>[2x]YYDYDHGSLGEPIRGVNIGGWLLLEPYITPSLFEAFRTNDDNDEGIPVDEYHFCQYLGKDLAKSRLQSHWSTFYQEQDFANIASQGFNLVRIPIGYWAFQILDDDPYVSGLQESYLDQAIGWARNNSLKVWVDLHGAAGSQN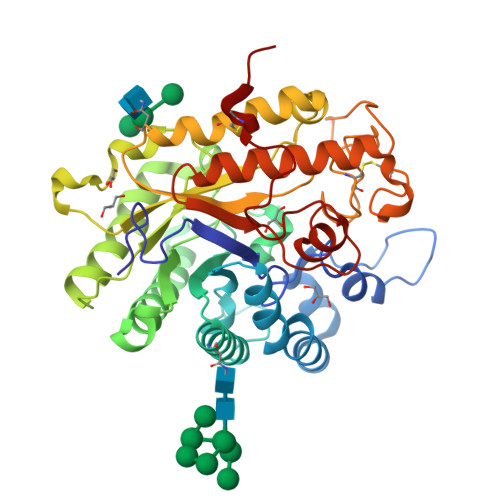GFDNSGLRDSYKFLEDSNLAVTINVLNYILKKYSAEEYLDIVIGIELINEPLGPVLDMDKMKNDYLAPAYEYLRNNIKSDQVIIIHDAFQPYNYWDDFMTENDGYWGVTIDHHHYQVFASDQLERSIDEHIKVACEWGTGVLNESHWIVCGEFAAALTDCIKWLNSVGFGARYDGSWVNGDQTSSYIGSCANNDDIAYWSDERKENTRRYVEAQLDAFEMRGGWIIWCYKTESSLEWDAQRLMFNGLFPQPLTDRKYPNQCGTISN> GASAPMVKIYTKNGDKGQTRIIGKQILYKNDPRVAAYGEVDELNSWVGYTKSLINSHTQVLSNELEEIQQLLFDCGHDLATPADDERHSFKFKQEQPTVWLEEKIDNYTQVVPAVKKFILPGGTQLASALHVARTITRRAERQIVQLMREEQINQDVLIFINRLSDYFF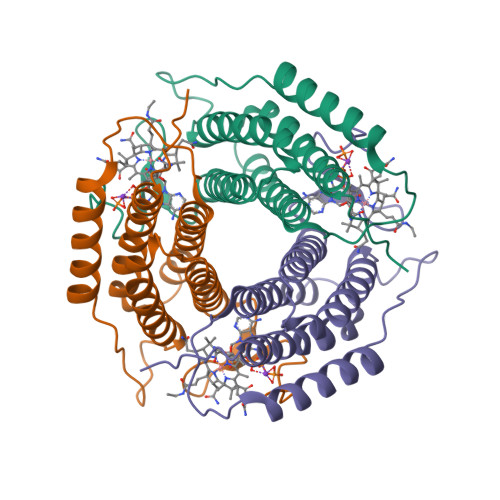AAARYANYLEQQPDMLYR> SNAMKISTKGRYGLTLMISLAKKEGQGCISLKSIAEENNLSDLYLEQLVGPLRNAGLIRSVRGAKGGYQLRVPAEEISAGDIIRLLEGPITFVESIESEPPAQKQLWIRMRDAVRDVLDNTTLKYLAEYVDTSEDLDG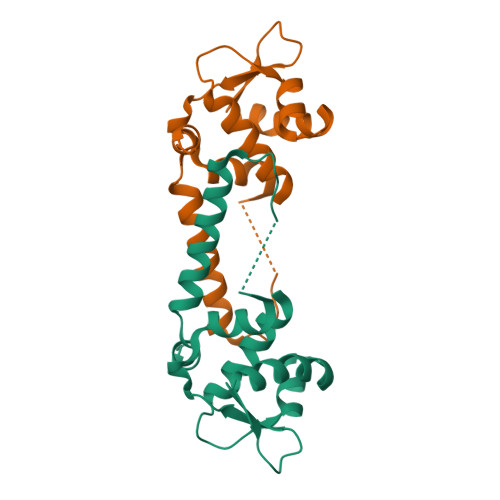YMFYI>[2x]STAGKVIKCKAAVLWEEKKP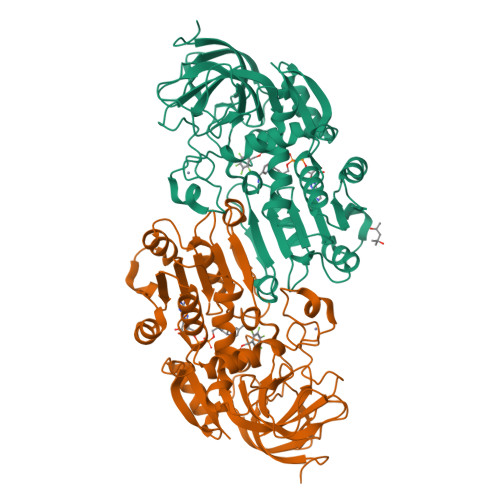FSIEEVEVAPPKAHEVRIKMVATGICRSDDQVVSGTLVTPLPVIAGHEAAGIVESIGEGVTTVRPGDKVIPLFTPQCGKCRVCKHPEGNFCLKNDLSMPRGTMQDGTSRFTCRGKPIHHFLGTSTFSQYTVVDEISVAKIDAASPLEKVCLIGCGFSTGYGSAVKVAKVTQGSTCAVFGLGGVGLSVIMGCKAAGAARIIGVDINKDKFAKAKEVGATECVNPQDYKKPIQEVLTEMSNGGVDFSFEVIGRLDTMVTALSCCQEAYGVSVIVGVPPDSQNLSMNPMLLLSGRTWKGAIFGGFKSKDSVPKLVADFMAKKFALDPLITHVLPFEKINEGFDLLRSGESIRTILTF Potassium‐coupled chloride transporters (KCCs) play crucial roles in regulating cell volume and intracellular chloride concentration. They are characteristically inhibited under isotonic conditions via phospho‐regulatory sites located within the cytoplasmic termini. Decreased inhibitory phosphorylation in response to hypotonic cell swelling stimulates transport activity, and dysfunction of this regulatory process has been associated with various human diseases. Here, we present cryo‐EM structures of human KCC3b and KCC1, revealing structural determinants for phospho‐regulation in both N‐ and C‐termini.

Due to preferred orientation of particles for KCC3, the map resolution for KCC3b‐WT was limited to 3.64 Å. While this structure was obtained under K+‐free conditions (Fig EV2A), we see the same configuration of the N‐terminus in a lower resolution structure of KCC3b‐PM in presence of K+ (Fig EV2D). By contrast, the maps of KCC3b‐WT, determined at 3.64 and 4.5 Å in detergent and MSP nanodiscs (Table 1 and Fig EV2B and C), do not show any electron density for the N‐terminal portion. On the other hand, there is no density for the N‐terminal helix in the cryo‐EM maps of KCC3b‐WT in both detergent (B) and nanodisc (C) environments. Because we see density for the N‐terminal segment only in the KCC3b‐PM mutant and not in the wild‐type KCC3b structure, we suspected that this configuration could be stabilized by a conformation of the CTD that brings the β5/α5 and β7/α6 loops into close proximity of the N‐terminus (Fig EV2G).

>[2x]MPHFTVTKVEDPEEGAAASISQEPSLADIKARIQDSDEPDLSQNSITGEHSQLLDDGHKKARNAYLNNSNYEEGDEYFDKNLALFEEEMDTRPKVSSLLNRMANYTNLTQGAKEHEEAENITEGKKKPTKTPQMGTFMGVYLPCLQNIFGVILFLRLTWVVGTAGVLQAFAIVLICCCCTMLTAISMSAIATNGVVPAGGSYFMISRALGPEFGGAVGLCFYLGTTFAAAMYILGAIEIFLVYIVPRAAIFHSDDALKESAAMLNNMRVYGTAFLVLMVLVVFIGVRYVNKFASLFLACVIVSILAIYAGAIKSSFAPPHFPVCMLGNRTLSSRHIDVCSKTKEINNMTVPSKLWGFFCNSSQFFNATCDEYFVHNNVTSIQGIPGLASGIITENLWSNYLPKGEIIEKPSAKSSDVLGSLNHEYVLVDITTSFTLLVGIFFPSVTGIMAGSNRSGDLKDAQKSIPIGTILAILTTSFVYLSNVVLFGACIEGVVLRDKFGDAVKGNLVVGTLSWPSPWVIVIGSFFSTCGAGLQSLTGAPRLLQAIAKDNIIPFLRVFGHSKANGEPTWALLLTAAIAELGILIASLDLVAPILSMFFLMCYLFVNLACALQTLLRTPNWRPRFRYYHWALSFMGMSICLALMFISSWYYAIVAMVIAGMIYKYIEYQGAEKEWGDGIRGLSLSAARFALLRLEEGPPHTKNWRPQLLVLLKLDEDLHVKHPRLLTFASQLKAGKGLTIVGSVIVGNFLENYGEALAAEQTIKHLMEAEKVKGFCQLVVAAKLREGISHLIQSCGLGGMKHNTVVMGWPNGWRQSEDARAWKTFIGTVRVTTAAHLALLVAKNISFFPSNVEQFSEGNIDVWWIVHDGGMLMLLPFLLKQHKVWRKCSIRIFTVAQLEDNSIQMKKDLATFLYHLRIEAEVEVVEMHDSDISAYTYERTLMMEQRSQMLRHMRLSKTERDREAQLVKDRNSMLRLTSIGSDEDEETETYQEKVHMTWTKDKYMASRGQKAKSMEGFQDLLNMRPDQSNVRRMHTAVKLNEVIVNKSHEAKLVLLNMPGPPRNPEGDENYMEFLEVLTEGLERVLLVRGGGSEVITIYS6-deoxy-6-sulfo-beta-D-glucopyranose | C6 H12 O8 S | 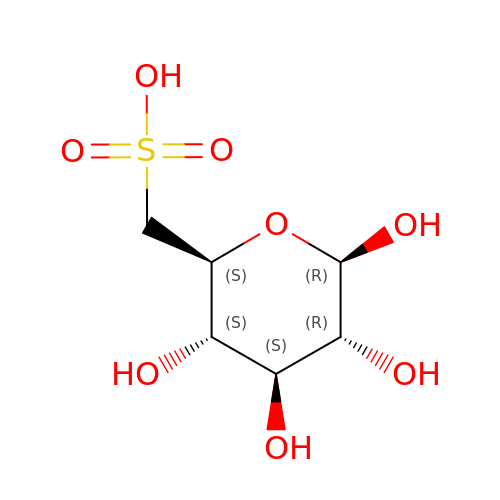QFBWOLBPVQLZEH-VFUOTHLCSA-N>RSMAEEVSTLMKATVLMRQPGRVQEIVGALRKGGGDRLQVISDFDMTLSRFAYNGKRCPSSYNILDNSKIISEECRKELTALLHHYYPIEIDPHRTVKEKLPHMVEWWTKAHNLLCQQKIQKFQIAQVVRESNAMLREGYKTFFNTLYHNNIPLFIFSAGIGDILEEIIRQMKVFHPNIHIVSNYMDFNEDGFLQGFKGQLIHTYNKNSSACENSGYFQQLEGKTNVILLGDSIGDLTMADGVPGVQNILKIGFLNDKVEERRERYMDSYDIVLEKDETLDVVNGLLQHILCQGVQLEMQGP[4x]

5’-Cytosolic nucleotidase IIIB (cN-IIIB) is one of the most recently discovered 5’-nucleotidases and has several unique structural and functional features. However, one of the most preferred cN-IIIB substrates is m7GMP, for which the activity of dephosphorylation is characterized by one order of magnitude lower KM constant compared to the other preferred substrates, whereas kcat/KM is comparable. The crystal structure of cN-IIIB consists of two distinct domains: the globular core domain (residues 1–51, 132–182, and 215–300) and the smaller CAP domain (52–131 and 183–214). The core domain is a haloacid dehalogenase domain (HAD).

Compound 5d’ is a decomposition product of 3,4-diFBn7GMP readily formed under crystallization conditions. Human cN-IIIB also efficiently accommodates N7-(3,4-diflorobenzyl)guanine (5d’) in its hydrophobic binding pocket. The crystal structure revealed that cN-IIIB binds 5d’ using the same hydrophobic moieties as in the case of 5d; however, the aromatic rings of 5d’ are reversely oriented compared to 5d. For 5d’, the guanine ring is accommodated in the hydrophobic cavity, where it is stabilized by hydrogen bonds between N1 and N2 and carboxylate group of Asp64. The guanine moiety participates in additional water-mediated interactions with a side chain of His 100 and backbone carbonyl of Ala157. The 3,4-difluorobenzyl moiety stacks in centered-parallel orientation between Trp105 and Tyr60, while the guanine ring is in edge-to-face stacking contact with Tyr60. In the complex structure of cN-IIIB • Mg2+ with 5d’ solved with 1.56 Å resolution, two additional electron densities were observed. The first one with tetrahedral shape belonged to the phosphate group, while an extensive analysis of the shape of second electron density revealed the structure of D-ribulose, which is likely formed during decomposition of 5d. The distance of < 1.5 Å between D-ribulose and oxygen of Glu88 carboxylic group indicates a covalent linkage between the molecules. Significant movement under ligand binding is also visible for the sidechain of Glu88, which forms hydrogen bonds to ribose moiety in 5d or covalent link to D-ribulose in the case of 5d’.> XXXXXXXXXXXXXXXKMPEWAACLSEIMKYNPKAVSELKHPLPHMSFVTFFVPFLLFAQERMSKAFSEFEKQEGGLSGIIDAAGYQDGIMSELHQCLDKLATRTLITELNVAREDGRLKGASPEERYVYFVEQYISDPEIYREFFELYPVLGRLMAEKVLRVLEIHEEIIGRFLSDRSLIAKKFNIASPELVGFEGDLGDSHKNGQSVKVLVLNNGKLVYKPRSLSIDEHYRELLNWLNGRGMKYSLRAAEVLDRGNYGWQEFVKHEGCSSEEELERFYFRQGGHLAILYGLRSVDFHNENIIASGEHPILIDLETLFDNHVSIFAQNQNLHVTALELKHSVLSSMMLPVKFKHDEVLDFDLSGIGGKGGQQSKKAKGYAVLNYGEDRMSLKETSLTTEEKLNAPKLNGRPVSAVFYTDFIVEGFKNAYAIMMKHKEELAGPSGFLNLFKHDEVRHVFRPTHVYGKFLEASTHPDYLTAGDKREQLFDYMWMLAKQSEKANVFIPDEIVDLL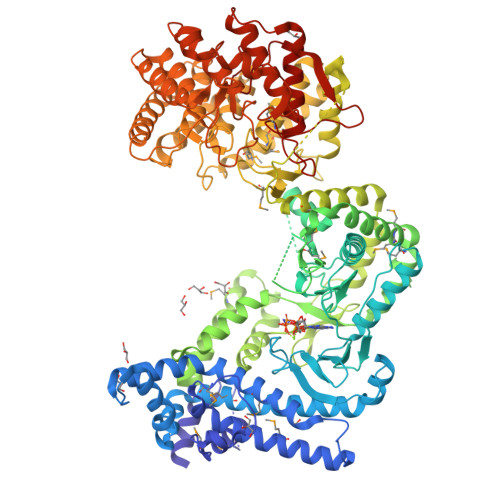LHDIPYFTFYAGGASLLNSRGEESEGFYETSSIDLAKKKIQSFSEKDLNHQLRYISLSMATLIENVWDHAESGLGQKETVADLGKEVKHIADDLLQKAIYSERGEGPFWISNNAGDEKMVFLSPLPMGLYDGMAGLAIFFAQAGKVLNEQVYTDTARSMIEEIQKEESYWVQNGNSHSAFFGTGSFIYLYSYLGSLWEDDSLLERALNLIPRVLDQPNQTQNPDFIAGDSGLLTVLVNLYEIKQHPAVLDSIRQVLSRLNDRIGRLLDSIEQDAVSLTGFSHGLTGIAFSIAKAAKVIHDDSCKELVLKLVEEEDRYFQKDHLNWLDLRNDSHTLSPSYWCHGAPGILLGRAHIQAFIPELTTRTLKLQEALQSSLNLADCQNHSLCHGLIGNLNILLDIKRLNRELHVPDDIFCIYKTKNRGWKTGLHSDVESLGMFVGTAGIAYGLLRLLDESVPSVLTLDIPTG> MRFWPFSKT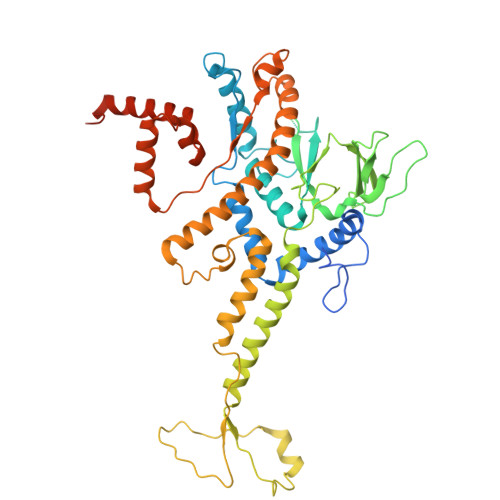TNAATRAEPMVTRPDTAPRVRSYRAAKSDRIAGGFGVFPTTPRDELRREIRGLVGHSRHAAQNFDYARAYEMLTRRHVIGFNGIRLQMDVRDPGGKKDVAAGAQIESAWARWGKMKNSPTPCGRLSWWGVECQVATGIAREGGSFVRIHQGTNRGRFGFQVEPIPFDLLDLDLTGPTPGGGFVGIAREGGSFVRIHQGTNRGRFGFQVEPIPFDLLDLDLTGPTPGGGFVESGVEFDATDRVVAYHMWSAAMSEGHRPGARRRLRIPAAQMLYVLVPEEIGQALGVPRSATALRLMNLSEKFQESALTAANYGASNMVFFERAADNGVVTGPEDDAQIPIDQIEAGTLTELPPGVKAVSHNPAYPDAAVGPFLRQMGTSQAAGLGVSYETLTADLSGANFSSLRAGKGEEREEWRMLQRAVFEGLHDRVFSRWLPLAMLSGEVRLPLAKLDKFDAATWRPRGWPSVNPKDDATAHEKDLKNGVRTRTEICAERGRDFADVVAEAAAERQMMRDAGLDPDAPLRTSPPETPPDPGEEIEGKDT1-[3-azanyl-6-(2-hydroxyphenyl)pyridazin-4-yl]piperidin-4-ol 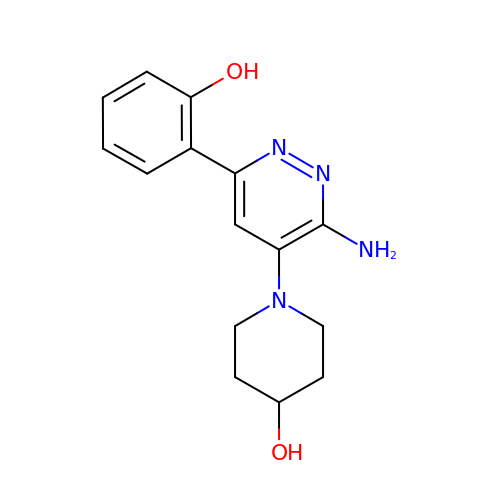| C15 H18 N4 O2 | IYHIMSKJSRZGKN-UHFFFAOYSA-N> GGA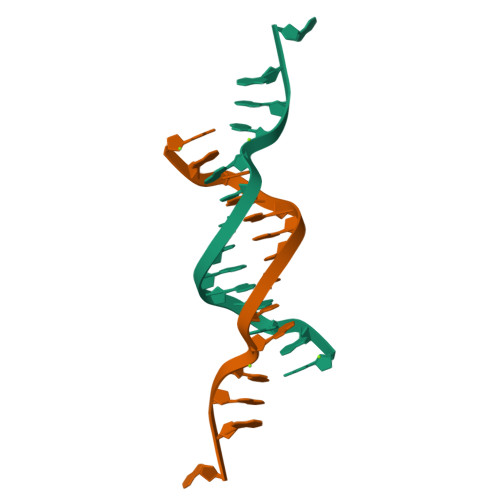AAGCTTGGAGA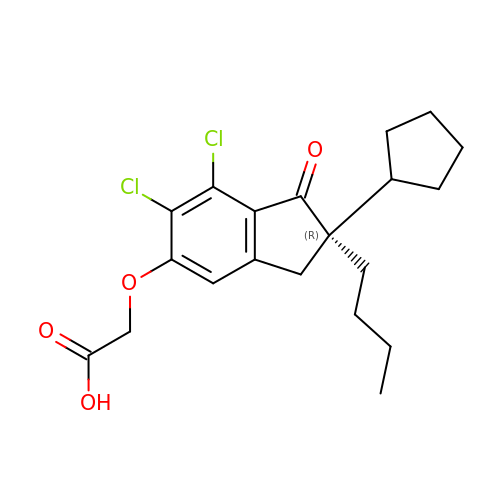2-[[(2~{R})-2-butyl-6,7-bis(chloranyl)-2-cyclopentyl-1-oxidanylidene-3~{H}-inden-5-yl]oxy]ethanoic acid | C20 H24 Cl2 O4 | YAWWQIFONIPBKT-HXUWFJFHSA-N> MEIQDYTDSEFKHALARNLRSLTRGKKSSKQPIAILLGGQSGAGKTTIHRIKQKEFQGNIVIIDGDSFRSQHPHYLELQQEYGKDSVEYTKDFAGKMVESLVTKLSSLGYNLLIEGTLRTVDVPKKTAQLLKNKGYEVQLALIATKPELSYLSTLIRY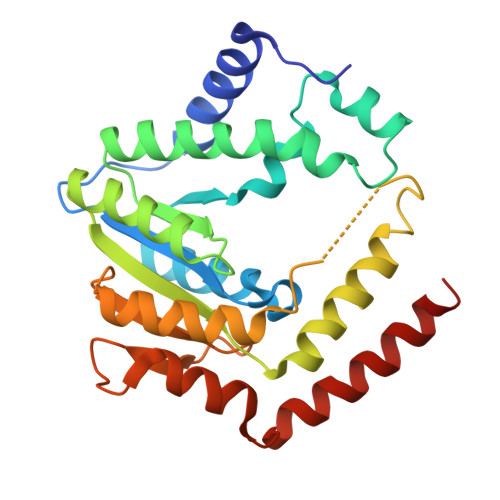EELYIINPNQARATPKEHHDFIVNHLVDNTRKLEELAIFERIQIYQRDRSCVYDSKENTTSAADVLQELFFGEWSQVEKEMLQVGEKRLNELLEK>[4x]AECSVDIQGNDQMQFNTNAITVDKSCKQFTVN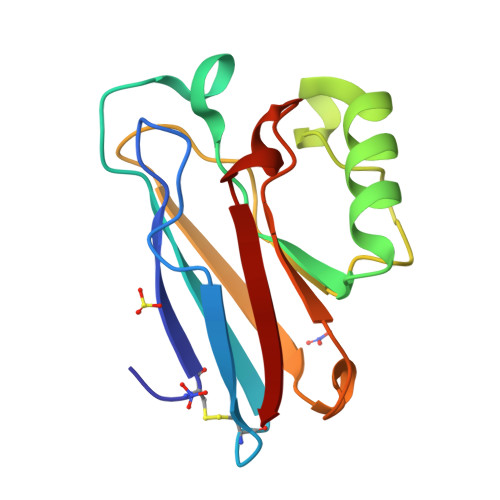LSHPGNLPKNVMGHNWVLSTAADMQGVVTDGMASGLDKDYLKPDDSRVIAHTKLIGSGEKDSVTFDVSKLKEGEQYMFFCTFPGHSALEKGTLTLK> SRKKMGLLVMAYGTPYKEEDIERYYTHIRRGRKPEPEMLQDLKDRYEAIGGISPLAQITEQQAHNLEQHLNEIQDEITFKAYIGLKHIEPFIEDAVAEMHKDGITEAVSIVLAPHFSTFSVQSYNKRAKEEAEKLGGLTITSVESWYDEPKFVTYWVDRVKETYASMPEDERENAMLIVSAHSLPEKI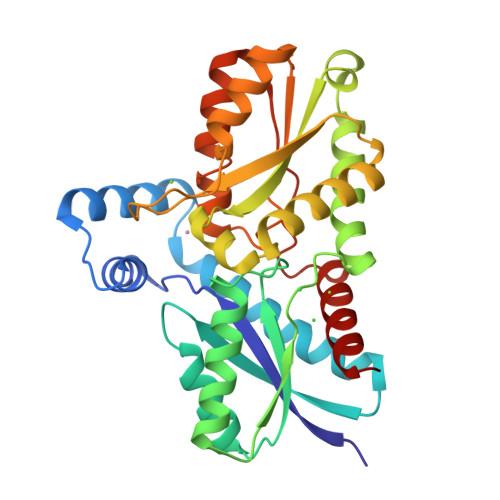KEFGDPYPDQLHESAKLIAEGAGVSEYAVGWQSEGNTPDPWLGPDVQDLTRDLFEQKGYQAFVYVPVGFVADHLEVLYDNDYECKVVTDDIGASYYRPEMPNAKPEFIDALATVVLKKLGR>MQLTRLVQVDCPL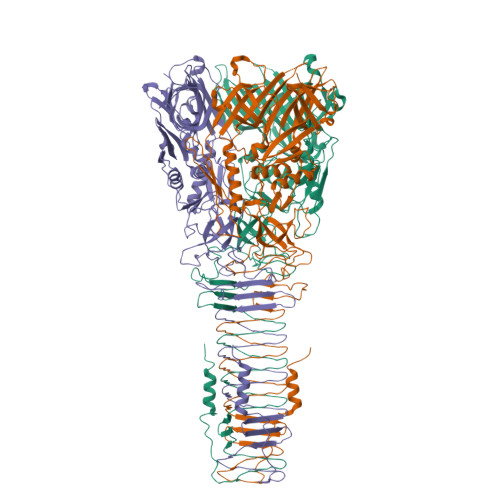GPDVLLLQRMEGREELGRLFAYELHLVSENPNLPLEQLLGKPMSLSLELPGGSRRFFHGIVARCSQVAGHGQFAGYQATLRPWPWLLTRTSDCRIFQNQSVPEIIKQVFRNLGFSDFEDALTRPYREWEYCVQYRETSFDFISRLMEQEGIYYWFRHEQKRHILVLSDAYGAHRSPGGYASVPYYPPTLGHRERDHFFDWQMAREVQPGSLTLNDYDFQRPGARLEVRSNIARPHAAADYPLYDYPGEYVQSQDGEQYARNRIEAIQAQHERVRLRGVVRGIGAGHLFRLSGYPRDDQNREYLVVGAEYRVVQELYETGSGGAGSQFESELDCIDASQSFRLLPQTPVPVVRGPQTAVVVGPKGEEIWTDQYGRVKVHFHWDRHDQSNENSSCWIRVSQAWAGKNWGSMQIPRIGQEVIVSFLEGDPDRPIITGRVYNAEQTVPYELPANATQSGMKSRSSKGGTPANFNEIRMEDKKGAEQLYIHAERNQDNLVENDASLSVGHDRNKSIGHDELARIGNNRTRAVKLNDTLLVGGAKSDSVTGTYLIEAGAQIRLVCGKSVVEFNADGTINISGSAFNLYASGNGNIDTGGRLDLNSGGASEVDAKGKGVQGTIDGQVQAMFPPPAKG[3x]>[4x]MN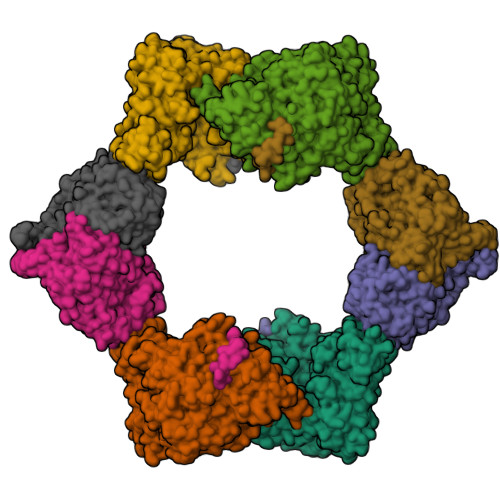QNLLVTKRDGSTERINLDKIHRVLDWAAEGLHNVSISQVELRSHIQFYDGIKTSDIHETIIKAAADLISRDAPDYQYLAARLAIFHLRKKAYGQFEPPALYDHVVKMVEMGKYDNHLLEDYTEEEFKQMDTFIDHDRDMTFSYAAVKQLEGKYLVQNRVTGEIYESAQFLYILVAACLFSNYPRETRLQYVKRFYDAVSTFKISLPTPIMSGVRTPTRQFSSCVLIECGDSLDSINATSSAIVKYVSQRAGIGINAGRIRALGSPIRGGEAFHTGCIPFYKHFQTAVKSCSQGGVRGGAATLFYPMWHLEVESLLVLKNNRGVEGNRVRHMDYGVQINKLMYTRLLKGEDITLFSPSDVPGLYDAFFADQEEFERLYTKYEKDDSIRKQRVKAVELFSLMMQERASTGRIYIQNVDHCNTHSPFDPAIAPVRQSNLCLEIALPTKPLNDVNDENGEIALCTLSAFNLGAINNLDELEELAILAVRALDALLDYQDYPIPAAKRGAMGRRTLGIGVINFAYYLAKHGKRYSDGSANNLTHKTFEAIQYYLLKASNELAKEQGACPWFNETTYAKGILPIDTYKKDLDTIANEPLHYDWEALRESIKTHGLRNSTLSALMPSETSSQISNATNGIEPPRGYVSIKASKDGILRQVVPDYEHLHDAYELLWEMPGNDGYLQLVGIMQKFIDQSISANTNYDPSRFPSGKVPMQQLLKDLLTAYKFGVKTLYYQNTRDGAEDAQDDLVPSIQDDGCESGACKI;>[4x]AYTTFSQTKNDQLKEPMFFGQPVNVARYDQQKYDIFEKLIEKQLSFFWRPEEVDVSRDRIDYQALPEHEKHIFISNLKYQTLLDSIQGRSPNVALLPLISIPELETWVETWAFSETIHSRSYTHIIRNIVNDPSVVFDDIVTNEQIQKRAEGISSYYDELIEMTSYWHLLGEGTHTVNGKTVTVSLRELKKKLYLCLMSVNALEAIRFYVSFACSFAFAERELMEGNAKIIRLIARDEALHLTGTQHMLNLLRSGADDPEMAEIAEECKQECYDLFVQAAQQEKDWADYLFRDGSMIGLNKDILCQYVEYITNIRMQAVGLDLPFQTRSNPIPWINTWLVSDNVQVAPQEVEVSSYLVGQIDSEVDTDDLSNFQL(6~{R},7~{R},9~{E})-6,7-bis(oxidanyl)hexadeca-9,15-dien-11,13-diynoic 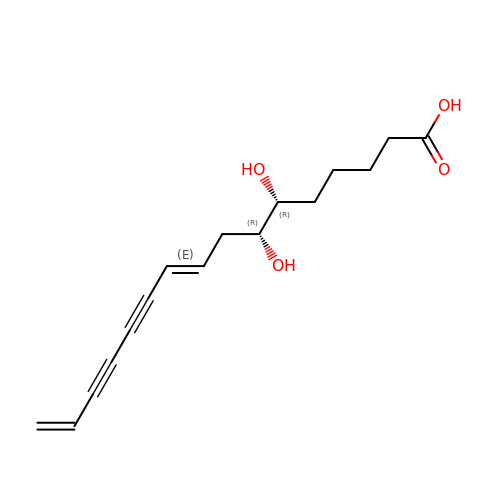acid | C16 H20 O4 | JBBDMFIFQBMXHD-FHFZEBMASA-N>GGSAIGELVRYLNTNPVGGLLEYARSHGFAAEFKLVDQSGPPHEPKFVYQAKVGGRWFPAVCAHSKKQGKQEAADAAL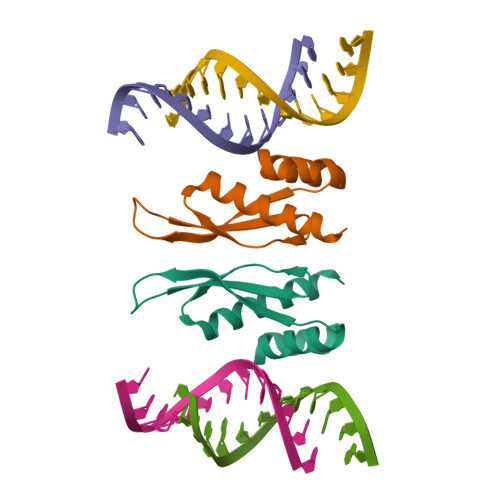RVLIGENE[2x]1-[3-(4-chlorophenoxy)propyl]-1H-imidazole 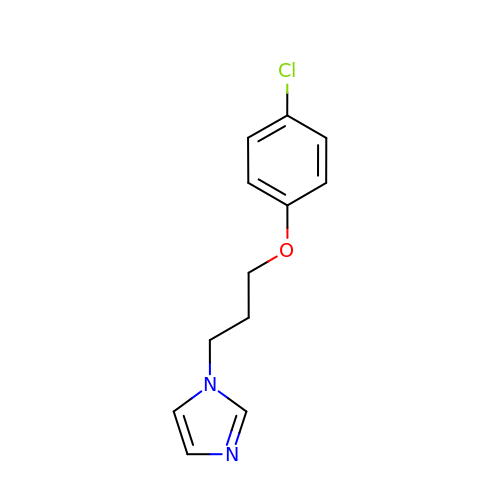| C12 H13 Cl N2 O | SKSDKBJVBWKTMH-UHFFFAOYSA-N>GKLEARAALNQALEMKRQGKREKAQKLFMHALKMDPDFVDALTEFGIFSEEDKDIIQADYLYTRALTISPYHEKALVNRDRTLPLVEEIDQRYFSIIDSKVKKVMSIPKGNSALRRVMEETYYHHIYHTVAIGGNTLTLSEIRHILETRYAVPGKSLEEQNEVIGMHAAMKYINTTLVSRIGSVTISDVLEIHRRVLGYVDPVEAGRFRTTQVLVGHHIPPHPQDVEKQMQEFVQWLNSEEAMNLHPVEFAALAHYKLVYIHPFIDGNGRTSRLLMNLILMQ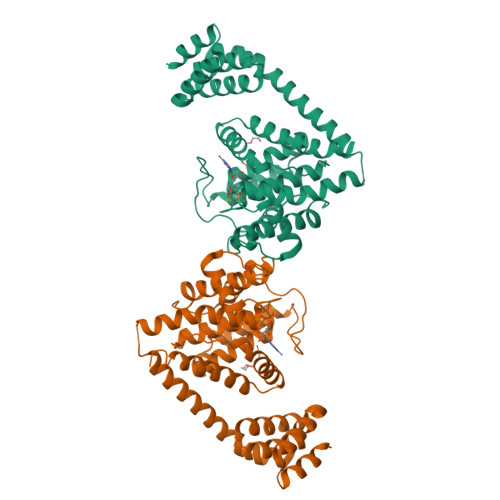AGYPPITIRKEQRSDYYHVLEAANEGDVRPFIRFIAKCTETTLDTLLFATTEYSVALPEAQP[2x]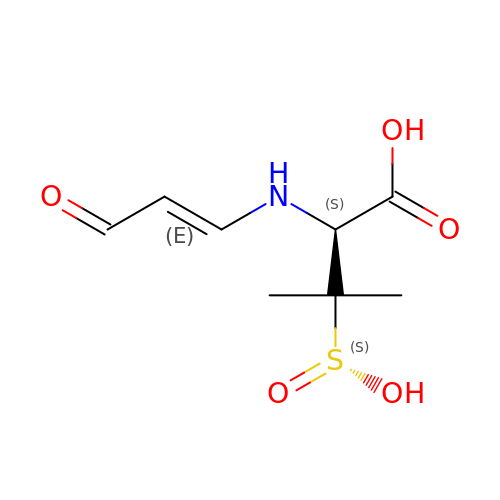TRANS-ENAMINE INTERMEDIATE OF SULBACTAM | C8 H13 N O5 S | DPHUOYJKDIRKGT-YUDCMIJISA-N>[2x]MRVEGAIGKTPVVRLAKVVEPDMAEVWVKLEGLNPGGSIKDRPAWYMIKDAEERGILRPGSGQVIVEPTSGNTGIGLAMIAASRGYRLILTMPAQMSEERKRVLKAFGAELVLTDPERRMLAAREEALRLKEELGAFMPDQFKNPANVRAHYETTGPELYEALEGRIDAFVYGSGTGGTITGVGRYLKERIPHVKVIAVEPARSNVLSGGKMGQHGFQGMGPGFIPENLDLSLLDGVIQ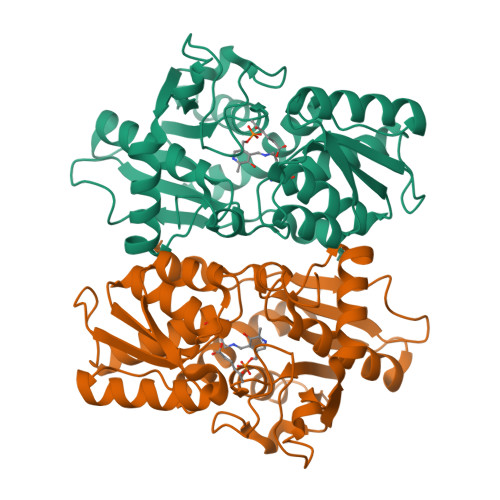VWEEDAFPLARRLAREEGLFLGMSSGGIVWAALQVARELGPGKRVACISPDGGWKYLSTPLYAEP> MGSSHHHHHHSQDPMGQVLPLVTRQGDRIAIVSGLRTPFARQATAFHGIPAVDLGKMVVGELLARSEIPAEVIEQLVFGQVVQMPEAPNIAREIVLGTGMNVHTDAYSVSRACATSFQAVANVAESLMAGTIRAGIAGGADSSSVLPIGVSKKLARVLVDVNKARTMSQRLKLFSRLRLRDLMPVPPAVAEYSTGLRMGDTAEQMAKTYG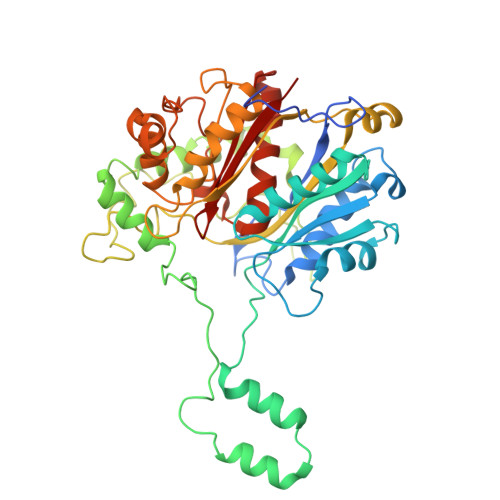ITREQQDALAHRSHQRAAQAWSDGKLKEEVMTAFIPPYKQPLVEDNNIRGNSSLADYAKLRPAFDRKHGTVTAANSTPLTDGAAAVILMTESRAKELGLVPLGYLRSYAFTAIDVWQDMLLGPAWSTPLALERAGLTMSDLTLIDMHEAFAAQTLANIQLLGSERFAREALGRAHATGEVDDSKFNVLGGSIAYGHPFAATGARMITQTLHELRRRGGGFGLVTACAAGGLGAAMVLEAE>MSNPSLVIVSPALPGANNGNWRTAQRWKALLSPVCSARVVQQWPDADASADTVMLALHARRSAESIAHWAHAHPGRGLGVVLTGTDLYQDIGSDPQAQRSLQLAQRLVVLQALGAEALPPECRAKARVVYQSTSARAELPKSARQLRAVM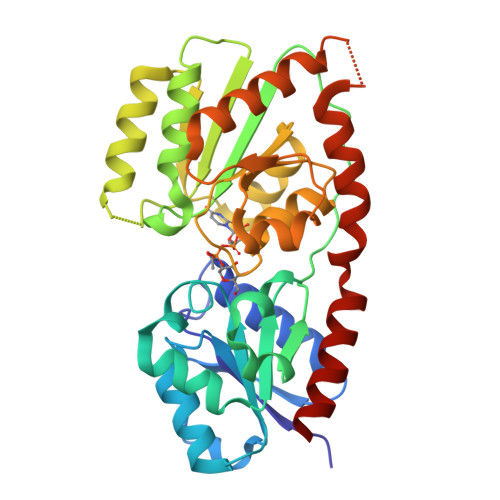VGHLRQVKSPQTLFDAARLLCGREDIRIDHIGDAGDAGLGELARALASDCPGYRWLGALPHAQTRQRIQRAHVLVHTSALEGGAHVIMEAVRSGTPVLASRVPGNVGMLGNDYAGYFPHGDAAALAALLEACRAGQGSKDRAAGLLDSLRTQCALRAPLFDPRAEQAALFQLLNELQPPPP[3x]>MNPETMNENGKSLKILFTALFGPGHLNACLGIGSLLRKRGHQIYFAHFPRHRATIEKHGFLFISLLDYAEPEFPIVDMLPDIGIIAKFAFERMHKLTPLELFRHASGKHTFAGMVNGSKGENYAMMKIVKEYKPDVCLADYLFNMPWMFTVDCPVIPVKSVNPIELYNGPPALTGCSIHDPPSVREEIEQLARKSELELESELEKLFAHFNVPLVSYNYAQQLGIYIYPGPLDYKELGSPKENWVRLDSSIRSTEISNFELPEKLKDKPGKLIYVSMGSLASAVTELLTMILTPLANSPHRFIVSTGPN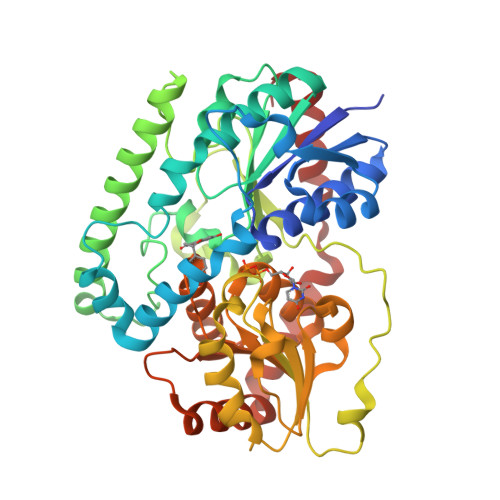GDSIKLYDNMWGDKFINQVALLPKVDLFITHGGSNSLIEGLTAGKPLIAIPQFGDQLDNAQRIADLGLGVRLNLHEFSGEKLLKAIEDVLNDEKINANVARVSEELKKSDSKDKVISLIEKLARDKKL[2x]(2~{S})-1-[(2~{R})-2-azanyl-3-phenyl-propanoyl]-~{N}-[[2,6-bis(azanyl)pyridin-4-yl]methyl]pyrrolidine-2-carboxamide 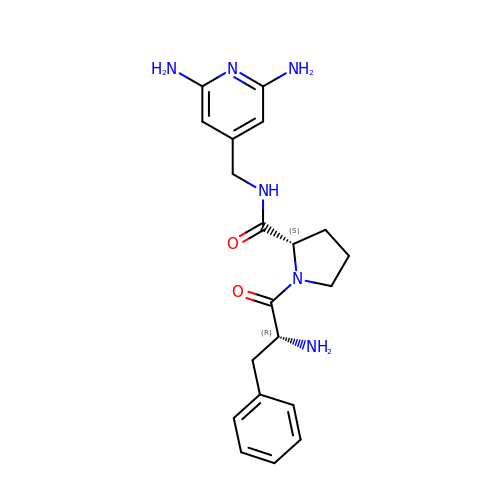| C20 H26 N6 O2 | ULOXRVUIRNGIOC-CVEARBPZSA-N>MSPRKTYILKLYVAGNTPNSVRALKTLKNILEVEFQGVYALKVIDVLKNPQLAEEDKILATPTL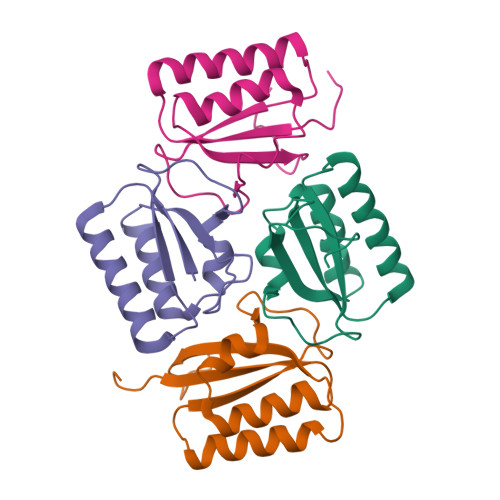AKVLPLPVRRIIGDLSDREKVLIGLDLLYGELQDSDDF[4x]(2R,3S,5R)-2-(2,5-difluorophenyl)-5-(7H-pyrrolo[3',4':3,4]pyrazolo[1,5-a]pyrimidin-8(9H)-yl)oxan-3-amine 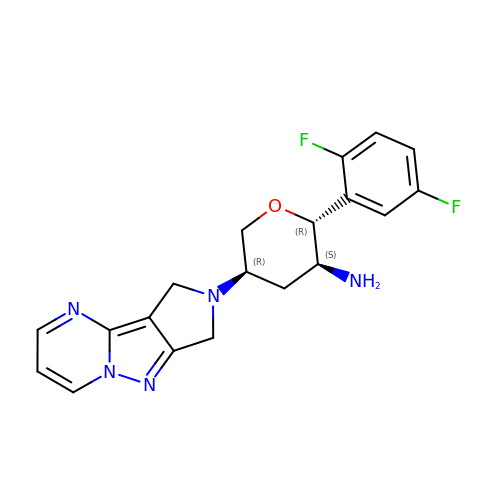| C19 H19 F2 N5 O | CEOQJSZJQDMDFU-PZPSRYQVSA-N>[5x]NPGGFGNQGGFGNSRGGGAGLGNNQGSNMGGGMNFGAFSINPAMMAAAQAALQSSWGMMGMLASQQNQSGPSGNNQNQGNMQ

TDP-43 is the primary component of the cytoplasmic inclusions in ~97% of ALS and ~45% of FTLD (that is, FTLD-TDP) cases. Full-length TDP-43 (FL TDP-43) consists of 414 amino acids with two RNA recognition motifs (RRM1 (105–169) and RRM2 (193–253)) flanked by an N-terminal domain (NTD (1–80)) and C-terminal domain (CTD (277–414)). The folded domains of RRMs bind specifically to the UG-repeats of RNA and the TG-repeats of DNA and play an important role in TDP-43 function in transcription regulation. We show that TDP-43 filaments contain a β-sheet-rich helical amyloid core that is fully buried by the flanking structured domains of the protein.

Based on the abundance of peptides with respect to the spectral counts containing at least two repeats, we identified that the 82 amino acids containing core peptide (CP) regions between 279 and 360 likely formed the amyloid core of TDP-43. Under the same in vitro aggregation conditions used for the FL TDP-43, CP formed ThT-positive β-sheet-rich fibrils of different morphologies. Consistent with the negative-stain EM data, the cryo-EM analysis showed polymorphic CP fibrils exhibiting variable length as well as a tendency to undergo lateral associations. A combination of three-dimensional (3D) classification and structural refinement revealed two populations of ~70-Å CP fibrils. The first CP fibril population was reconstructed to 4.1-Å resolution and was composed of a single CP protofilament with stacked subunits along the fibril axis with a helical rise of 4.86 Å and a helical twist of −3.12°. The second CP fibril population was reconstructed to 3.7-Å resolution and revealed two protofilaments, which were non-identical with stacked subunits along the fibril axis with a helical rise of 4.83 Å and a helical twist of −3.09°. The atomic model was built from residues Gly281 to Gly351 into the most resolved density corresponding to the CP fibrils of one protofilament. The density of the second protofilament was mostly disordered, with disconnected loops, and was not used for model building. One cross-sectional layer of the atomic model revealed a novel ‘H-fold’ conformation of the CP filaments that consists of six linked β-strands with rigid loops and turns. Despite their similar sequence, the recombinant peptide 279–360 exhibited a very distinct fold with major differences in secondary structures (β-strands, turns and loops), in comparison with the core amyloid structure of brain-derived TDP-43 filaments or TDP-43 fibrils produced in vitro from the entire CTD domain or shorter CTD-derived peptide fragments.2-fluoranyl-4-[2-(4-hydroxyphenyl)propan-2-yl]phenol | 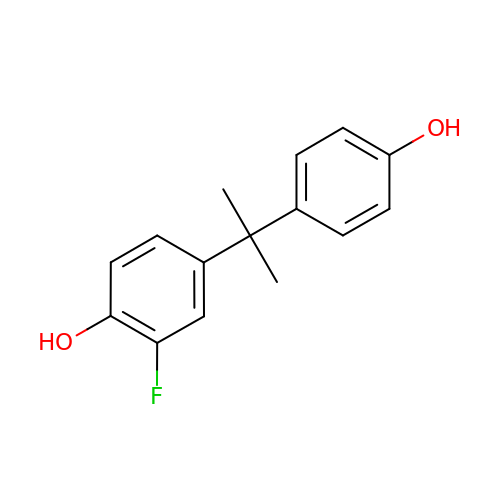C15 H15 F O2 | XMEGCBLYVCFWLJ-UHFFFAOYSA-N> MDTLFDAPGRSQFVPADQAFAFDFQQNQHDLNLTWQIKDGYYLYRKQIRITPEHAKIADVQLPQGVWH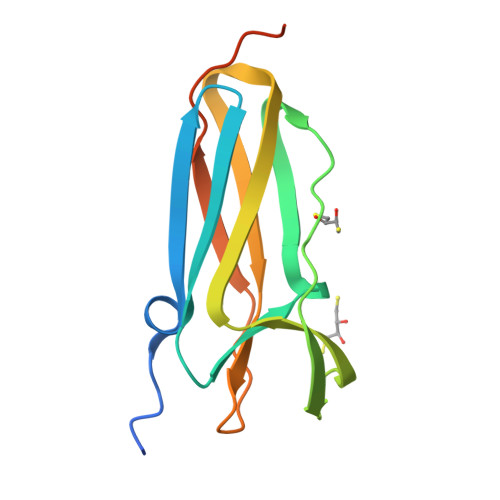EDEFYGKSEIYRDRLTLPVTINQASAGATLTVTYQGCADAGFCYPPETKTVPLSEVVANNAAPQPVGLVPR> HHHHHHMSSGKNAPKTGGGAKGNNASPAGSGNTKNNGASGADINNYAGQIKSAIESKFYDASSYAGKTCTLRIKLAPDGMLLDIKPEGGDPALCQAALAAAKLAKIPKPPSQAVYEV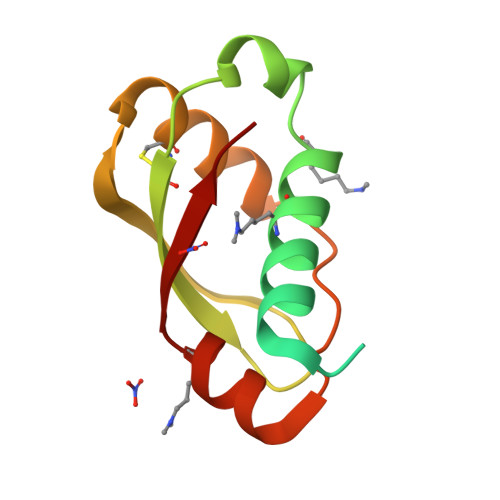FKNAPLDFKP> MIRFEQVGKRYPNGHVGLHEVSFRVHRGEILFVTGHSGAGKSTLLRLILAMERPTSGKLLLGGQDLGRITTAQIPFLRRQIGVVFQNHQLLTDRTVADNIALPLQILGMPKPEIAKRVASALERVNLKEKGEALPSDL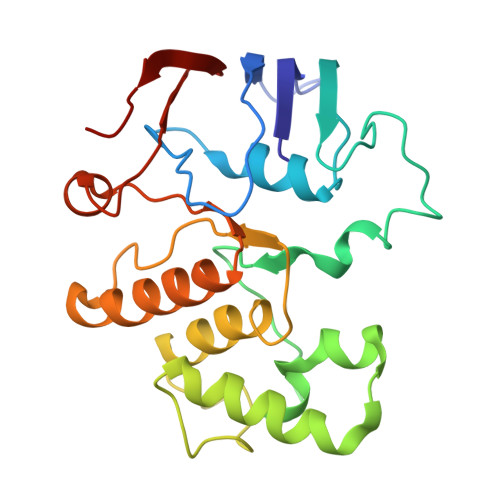STGQQQRVGIARAIVHQPALLLADEPTGNLDPRLASEIMGVFEDINRLGTTVLIASHDLALIARMRHRMLTLQRGRIIADREDEA> GSHMLSDEQMQIINSLVEAHHKTYDDSYSDFVRFRPPVREGPVTRSASRAASLHSLSDASSDSFNHSPESVDTKLNFSNLLMMYQDSGSPDSSEEDQQSRLSMLPHLADLVSYS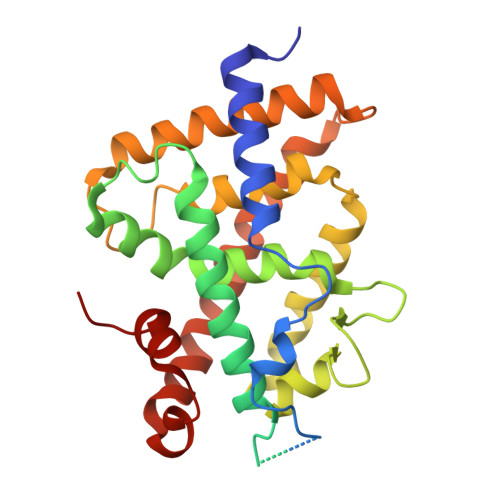IQKVIGFAKMIPGFRDLTAEDQIALLKSSAIEIIMLRSNQSFSLEDMSWSCGGPDFKYCINDVTKAGHTLEHLEPLVKFQVGLKKLKLHEEEHVLLMAICLLSPDRPGVQDHVRIEALQDRLCDVLQAYIRIQHPGGRLLYAKMIQKLADLRSLNEEHSKQYRSLSFQPEHSMQLTPLVLEVFGSEVS> MGTYRKRFNEKARSGHMAKLKELKRIRNKQFTRQDENDERVENPDSAPAESSTTEPNANAEILEPLTEEEKKMKKRKLQELFTPKESKVSRLKKKRLDKFIEHQLKREERKTIIGKLQDYKIDTSLLTSSKRLGEGRQTKKEEFKEALSLERQGRGNEQTNEILYEEYEPKVWDEYGEGGSSEDDDG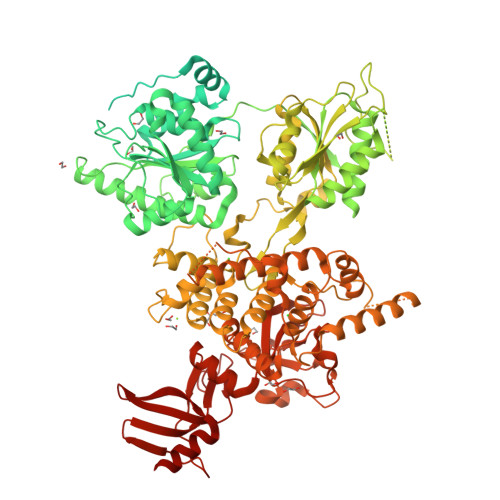EDDFEASFGSMPKPTDNEEKKSSGFIDHRPAKFGGSGLSFGFSNIKVINKESKTPKKKYNWRQRVEMEELKKHGKEDEMDFDTTSEDDDEEEDQEEEDKMHPSENPLEEVESADSETGSEKFDQNDVANEFKDWANQEIKKLEGRDQELVTPTLNIDYKPIIRKEDLDDGLQEAYVPINENSTRKAFYVEVSRSDEIQKARIQLPVFGEEHKIMEAIHHNDVVIICGETGSGKTTQVPQFLYEAGFGAEDSPDYPGMVGITQPRRVAAVSMAERVANELGDHGHKVGYQIRFDSTAKEDTKVKFMTDGVLLREMMHDFKLTKYSSIIIDEAHERNINTDILIGMLSRCVRLRAKLHKENPIEHKKLKLIIMSATLRVSDFSENKTLFPIAPPVLQVDARQFPVSIHFNRRTAFNYTDEAFRKTCKIHQKLPPGAILVFLTGQQEITHMVKRLRKEFPFKKNSKYNKDLETPVSKMGINSKTTDLEAEDIDFSVQVIDQDKFKSAIRYEEDEGNSGNGEDEEDEEEEGFEEVLTEGQTANDPLYVLPLYSLLPTKEQMRVFQKPPQGSRLCIVATNVAETSLTIPGVRYVVDSGRSKERKYNESNGVQSFEVGWVSKASANQRSGRAGRTGPGHCYRLYSSAVFEHDFEQFSKPEILRMPVESIVLQMKSMAIHNIINFPFPTPPDRVALSKAIQLLQYLGALDNKEMITEDGKKMSLFPLSPRFSKMLLVSDEKACLPYIVAIVSALSVGDPFINEFELGINEISRKPNPDENLDDKIREHDESTPGMDPELKKELRSKFYKSRSQFSKLDKFSDVFRLLSVVSAMDYVPKEQKEIFMKKNFLRGKLMEEIVKLRKQLMYIIKSNTSKENIAVVIRNEDLKSDIPSVIQIKLLKQMICAGFVDHVAVRADVLFPDDAKITNRTSIINIPYIPVLATRTPNIEDCFVYIHPTSILNNLGEMPPKYMLYYSLHLGGNNKTRMNTLCDIASTPLANIARKGLLLTYSKPLTGQGLKTVNLSPTERYCYVVPRFGSTVDNDLKIGWDLNPIAVHQKKQKGQWTVIKFITRKGFQTITGEEKEKK4-[2-(benzimidazol-1-yl)ethanoyl]-2-chloranyl-benzenesulfonamide | C15 H12 Cl N3 O3 S | 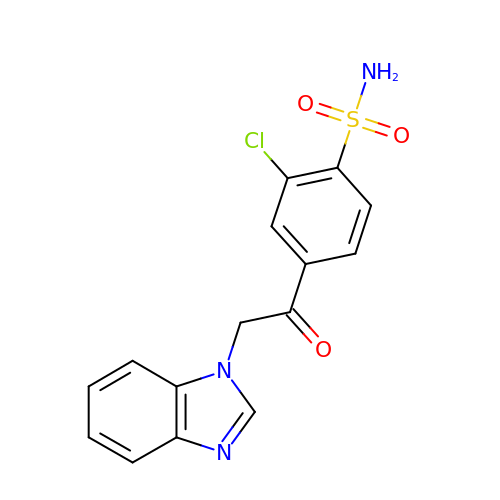SWJLGRBJIPSPCI-UHFFFAOYSA-N> DLHDKSELTDLALANAYGQYNHPFIKENIKSDEISGEKDLIFRNQGDSGNDLRVKFATADLAQKFKNKNVDIYGASFYYKCEKISENISECLYGGTTL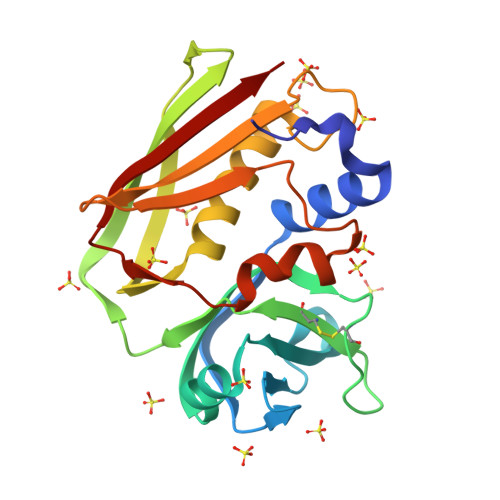NSEKLAQERVIGANVWVDGIQKETELIRTNKKNVTLQELDIKIRKILSDKYKIYYKDSEISKGLIEFDMKTPRDYSFDIYDLKGENDYEIDKIYEDNKTLKSDDISHIDVNLYT> 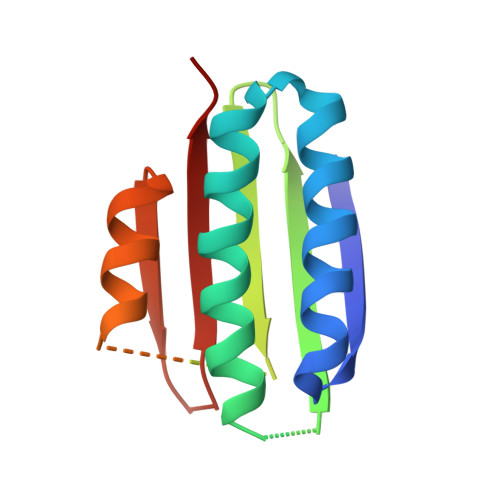ADYIEMKVPAQPEYVGIIRLTLSGVASRMGYTYDEIEDLKIAVSEACTNAVQHAYKEDKNGEVSIRFGVFEDRLEVIVADEGDSFDFDQKQQDLGPYTPSHTVDQLSEGGLGLYLMETLMDEVRVQNHSGVTVAMTKYLNG>[4x]SGGGDGSTYSAEIRRTTMGVPHIKAGNWGSAGYGFGYVQAQDNLCTMA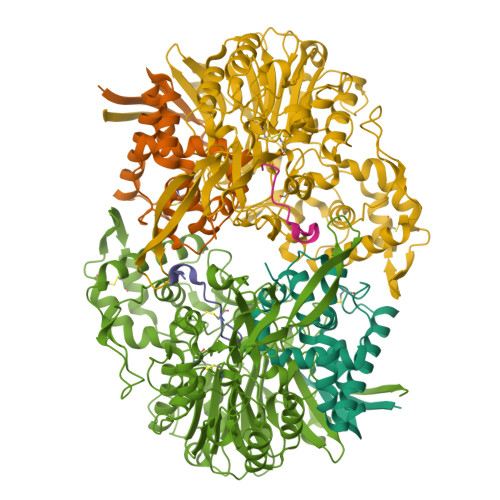DSFLTYRGERSRHLGGSAQLVYNSTLGRPRNIDSDFFHRHVISDEAVDRTMAAQPAKLLQMVEGFAAGYNRYVREAKAGGSAHAACRSEAWVQPITARDVWRRIYAANLAGGYSNFAEAIANAQPPQAKA;>GAQEPAAFEPGRTRAPSLQVGGELGVG[4x];>[4x]SNMYGFGTAATGEGSGVLFGNPHWYWKGPDRFYQAQLTIDGEANVSGVSFLGLPVIQIGFNDSVAWSHTVSTARRFGFFQLSLVQGEPTSYLRDGVPVKMKPATITVPSRNADGSVSDVTRTLYHSEFGPLVNLAGLNPALAWSQGTAFAIRDINGENFRTLRTWMRWNQAKSLDEFIAIQKEEASIPWVNTVAVGRGSAKAWYADIGAVPNVSPAQTAACTTPFGMAVGQALPNVPFFDGSRSECDWLTDADSVQKGAVGVSRMPSLQRDDYVGNMNDSYWLANVHAPLTGYPAIFGPAGTSAQTLRTRMGHTMALERLAGTDGYAGNKATSAVVREMVLGSRVFSAERFKDEVLDLICTPAQWTVNGAAVDAAQACAVLAAWDNRGRKDSRGSHLWDEFWSRVPTASLFTVPFSAADPLNTPRGINAAAADALRQAMATAIARVGQSGYALDAPRGEVLYATRGGTRLPLYGGCGAMGYFTITCSENDITQGGYSMDGQPNASNSYMQVVSFPASGVQAHTFLTFSLSDDPASPHHGDYTKAYSAGQWLRVPFTEAEITGNADYRTATVKELEHHHHHH>ELNRSQGIPFLEYKHFVTRTFFPKCSSLYEERYVLPSKTLNSQGGSPPQETHPLLGEWNIPEHCRPSMEEGISLFSSLLNNKHFLIVFVHALEQQKDFAVRDRCSLASLLTIALHGKLEYYTSIMKELLVDLIDASAAKNPKLMLRRTESVVEKMLTNWMSICMYGCLRETVGEPFFLLLCAIKQQINKGSIDAITGKARYTLNEEWLLRENIEAKPRNLNVSFQGCGMDSLSVRAMDTDTLTQVKEKILEAFCKNVPYSQWPRAEDVDLEW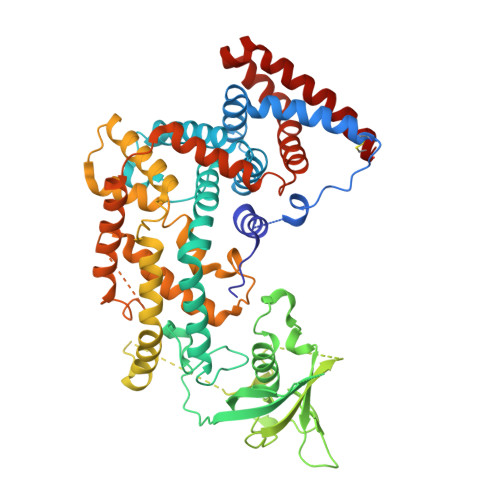FASSTQSYVLRDLDDTSVVEDGRKKLNTLAHYKIPEGASLAMSLTDKKDSTLGRVKDLDTEKYFHLVLPTDELVEPKKSHRQSHRKKVLPEIYLTRLLSTKGTLQKFLDDLFKAILSIREDKPPLAVKYFFDFLEEQAEKRGISDPDTLHIWKTNSLPLRFWVNILKNPQFVFDIEKTDHIDACLSVIAQAFIDACSISDLQLGKDSPTNKLLYAKEIPEYRKTVQRYYKQIQDMTPLSEQEMNAHLAEESRKYQNEFNTNVAMAEIYKYAKRYRPQIMAALEANPTARRTQLQHKFEQVVALMENNIYECYSEA[2x]>GVNPRGLGPLQIWQTDFTLEPRMAPRSWLAVTVDTASSAIVVTQHGRVTSVAVQHHWATAIAVLGRP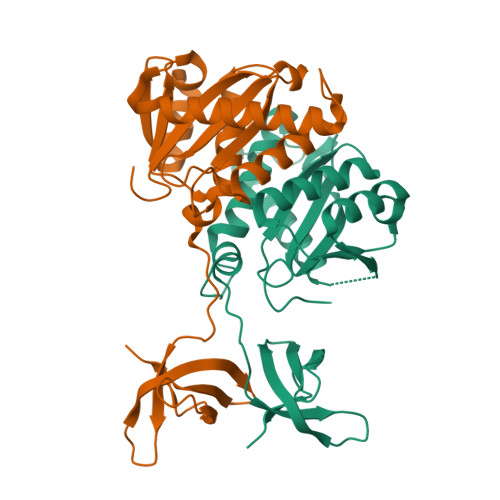KAIKTDNGDAFTSKSTREWLARWGIAHTTGIPGNSQGQAMVCRANRLLKDKIRVLAEGDGFMKRIPTSKQGELLAKAMYALNHKERGENTKTPIQKHWRPTVLTEGPPVKIRIETGEWEKGWNVLVWGRGYAAVKNRDTDKVIWVPSRKVKPDIT[2x]> MFENITAAPADPILGLADLFRADERPGKINLGIGVYKDETGKTPVLTSVKKAEQYLLENETTKNYLGIDGIPEFGRCTQELLFGKGSALINDKRARTAQTPGGTGALRVAADFLAKNTSVKRVWVSNPSWPNHKSVFNSAGLEVREYAYYDAENHTLDFDALINSLNEAQAGDVVLFHGCCHAPTGIDPTLEQWQTLAQLSVEKGWLPLFDFAYQGFARGLEEDAEGLRAFAAMHKELIVASSYSKNFGLYNERVGACTLVAADSETVDRAFSQMKAAILANYSNPPAHGASVVATILSNDALRAIWEQELTDMRQRIQRMRQLFVNTLQEKGANRDFSFIIKQNGMFSFSGLTKEQVLRLREEFGVY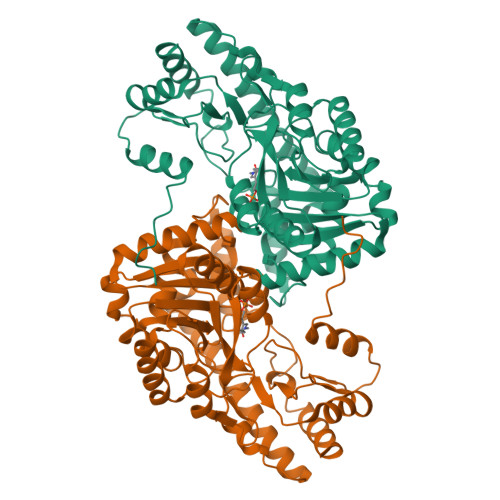AVASGRVNVAGMTPDNMAPLCEAIVAVL The β-fructofuranosidase (EC 3.2.1.26) from the ascomycetous yeast Schwanniomyces occidentalis (Ffase) is a robust glycoside hydrolase (GH) that releases fructose units from sucrose and inulin (hydrolytic activity) but also produced 6-kestose, 1-kestose, neokestose (all trisaccharides) and blastose (disaccharide) by transfructosylation of sucrose (transferase activity). Ffase is a butterfly-shaped homodimer of 160 KDa included in the GH family 32 (GH32). Each subunit of 535 amino acids presents a bimodular arrangement with a N-terminal five fold β-propeller catalytic domain and a C-terminal β-sandwich supplementary domain linked by a short residue segment. As with other β-fructofuranosides of the same family, Ffase performs its enzymatic action through a pair of key negatively-charged amino acids in its active site, namely, Asp-50 acting as a nucleophile and Glu-230 as an acid/base catalyst.

However, only sucrose was observed in crystals grown in the presence of fructosyl-mannitol, most probably due to traces of this disaccharide in the purified product. For its part, the glucose at + 1 is recognized through a complex net of direct and water-mediated polar linkages. First, there is a bifurcated hydrogen bond between both oxygens from the catalytic Glu-230 carboxylate to the O2 and O3 of glucose, these atoms in turn being also linked to Gln-228 and Asn-254 side-chains, respectively. Moreover, the glucose O4 is linked through two water molecules to Gln-147, Gln-176, and Gln-228. Consequently, the pair Gln-228/Asn-254, previously defined as a hotspot for regulating the transfructosylated product specificity, is also directly involved in the donor-sucrose binding, which necessarily must influence the first step of the enzymatic mechanism with alternative acceptors. Moreover, the Ffase-sucrose complex shows several long-chain residues in the environment of the catalytic Glu-230 that make a complicated network of polar linkages, keeping a tight architecture at this part of the catalytic site. Thus, in addition to Arg-178 at the conserved RPD motif, Gln-176 and Gln-228 are making an intricate polar net for keeping Glu-230 side-chain in a very precise conformation and for stabilizing the binding of sucrose. The complex Ffase-D50A/sucrose showed that the pair Gln-228/Asn-254 is additionally involved in donor substrate recognition by making direct hydrogen bonds with sucrose.

>MVQVLSVLVIPLLTLFFGYVASSSIDLSVDTSEYNRPLIHFTPEKGWMNAPNGLFYDKTAKLWHLYFQYNPNATAWGQPLYWGHATSNDLVHWDEHEIAIGPEHDNEGIFSGSIVVDHNNTSGFFNSSIDPNQRIVAIYTNNIPDNQTQDIAFSLDGGYTFTKYENNPVIDVSSNQFRDPKVFWHEDSNQWIMVVSKSQEYKIQIFGSANLKNWVLNSNFSSGYYGNQYECPGLIEVPIENSDKSKWVMFLAINPGSPLGGSINQYFVGDFDGFQFVPDDSQTRFVDIGKDFYAFQTFSEVEHGVLGLAWASNWQYADQVPTNPWRSSTSLARNYTLRYVHTNAETKQLTLIQNPVLPDSINVVDKLKKKNVKLTNKKPIKTNFKGSTGLFDFNITFKVLNLNVSPGKTHFDILINSQELNSSVDSIKIGFDSSQSSFYIDRHIPNVEFPRKQFFTDKLAAYLEPLDYDQDLRVFSLYGIVDKNIIELYFNDGTVAMTNTFFMGEGKYPHDIQIVTDTEEPLFELESVIIRELNK[2x]> MGDSFYIRTHFELEPSPPSGLGFTRGDVFHVLDTLHPGPGQSHARGGHWLAVRMGRDLREQERGIIPNQSRAEQLASLEA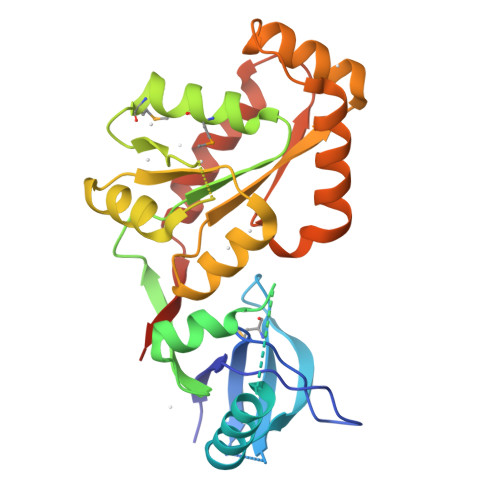AQRAVGVGPGSSAGSNARAEFWRLRGLRRGAKKTTQRSREDLSALTRQGRYPPYERVVLREASFKRPVVILGPVADIAMQKLTAEMPDQFEIAETVSRTDSPSKIIKLDTVRVIAEKDKHALLDVTPSAIERLNYVQYYPIVVFFIPESRPALKALRQWLAPASRRSTRRLYAQAQKLRKHSSHLFTATIPLNGTSDTWYQELKAIIREQQTRPIWTAEDQLHHHHHH> MSRSVLQPSQQKLAEKLTILNDRGVGMLTRLYNIKKACGDPKAKPSYLIDKNLESAVKFIVRKFPAVETRNNNQQLAQLQKEKSEILKNLALYYFTFVDVMEFKDHVCELLNTIDVCQVFFDITVNFDLTKNYLDLIITYTTLMILLSRIEERKAIIGLYNYAHEMTHGASDREYPRLGQMIVDYENPLKKMMEEFVPHSKSLSDALISLQMVYPRRNLSADQWRNAQLLSLISAPSTMLNPAQSDTMPCEYLSLDAMEKWIIFGFILCHGILNTDATALNLWKLALQSSSCLSLFRDEVFHIHKAAEDLFVNIRGYNKRINDIRECKEAAVSHAGSMHRERRKFLRSALKELATVLSDQPGLLGPKALFVFMALSFARDEIIWLLRHADNMPKKSADDFIDKHIAELIFYMEELRAHVRKYGPVMQRYYVQYLSGFDAVVLNELVQNLSVCPEDESIIMSSFVNTMTSLSVKQVEDGEVFDFRGMRLDWFRLQAYTSVSKASLGLADHRELGKMMNTIIFHTKMVDSLVEMLVETSDLSIFCFYSRAFEKMFQQCLELPSQSRYSIAFPLLCTHFMSCTHELCPEERHHIGDRSLSLCNMFLDEMAKQARNLITDICTEQCTLSDQLLPKHCAKTISQAVNKKSKKQTGKKGEPEREKPGVESMRKNRLVVTNLDKLHTALSELCFSINYVPNMVVWEHTFTPREYLTSHLEIRFTKSIVGMTMYNQATQEIAKPSELLTSVRAYMTVLQSIENYVQIDITRVFNNVLLQQTQHLDSHGEPTITSLYTNWYLETLLRQVSNGHIAYFPAMKAFVNLPTENELTFNAEEYSDISEMRSLSELLGPYGMKFLSESLMWHISSQVAELKKLVVENVDVLTQMRTSFDKPDQMAALFKRLSSVDSVLKRMTIIGVILSFRSLAQEALRDVLSYHIPFLVS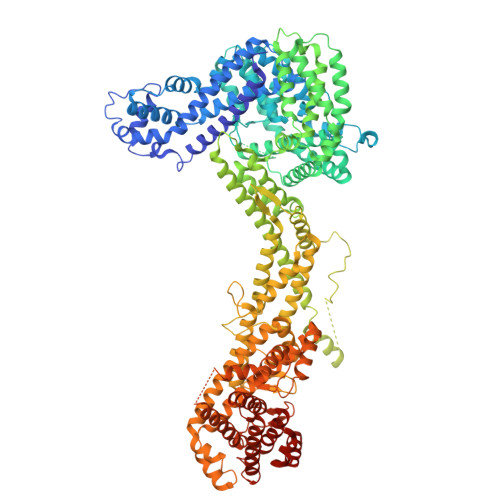SIEDFKDHIPRETDMKVAMNVYELSSAAGLPCEIDPALVVALSSQKSENISPEEEYKIACLLMVFVAVSLPTLASNVMSQYSPAIEGHCNNIHCLAKAINQIAAALFTIHKGSIEDRLKEFLALASSSLLKIGQETDKTTTRNRESVYLLLDMIVQESPFLTMDLLESCFPYVLLRNAYHAVYKQSVTSSA> GEIAAIKQEI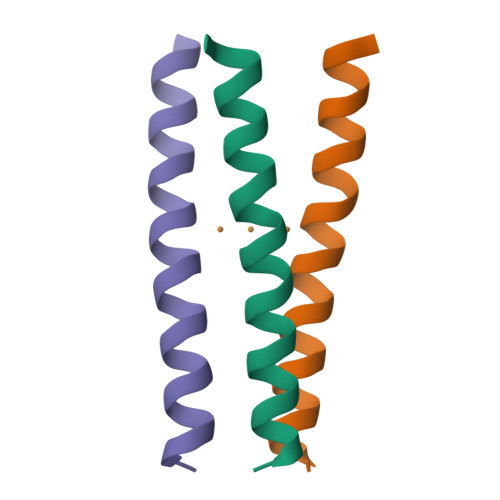AAHKKEHAAIKWEIAAIKQGYG>SNAMPLPKSLKYGDTIGIYSPSSPVTYTSPKRFERAKSYLLQKGFHILEGSLTGRYDYYRSGSIQERAKELN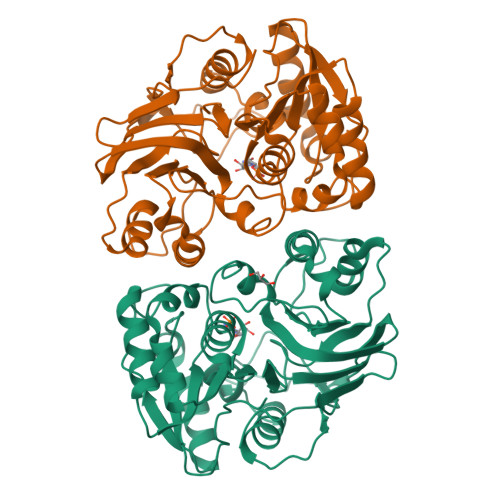ALIRNPNVSCIMSTIGGMNSNSLLPYIDYDAFQNNPKIMIGYADATALLLGIYAKTGIPTFYGPALVPSFGEFEPFVDDTYKYFLETLLHDQALPYNIKQPLFWSDEFINWEEKTKEKELRPNNWISVTNGQATGRVIGGNLNTIQGIWGSPYMPCIQEGDILFIEDSSKDAATIERSFSFLKINGVFDKVSGIILGKHEQFDDCGTNRKPYEILLEVLQNQRIPLLADFDCCHTHPMITMPIGVQVKMDATNKTIHILEKWKI[2x]>SFSQAVSGLNAAATNLDVIGNNIANSATYGFKSGTASFADMFAGSKVGLGVKVAGITQDFTDGTTTNTGRGLDVAISQNGFFRLVDSNGSVFYSRNGQFKLDENRNLVNMQGMQLTGYPATGTPPTIQQGANPAPITIPNTLMAAKSTTTASMQINLNSTDPVPSKTPFSVSDADSYNKKGTVTVYDSQGNAHDMNVYFVKTKDNEWAVYTHDSSDPAATAPTTASTTLKFNENGILESGGTVNITTGTINGATAATFSLSFLNSMQQNTGANNI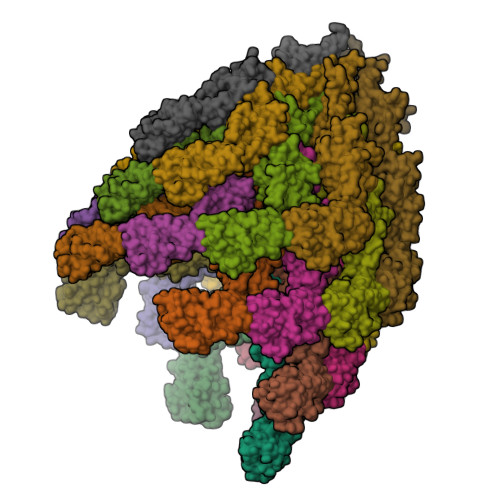VATNQNGYKPGDLVSYQINNDGTVVGNYSNEQEQVLGQIVLANFANNEGLASQGDNVWAATQASGVALLGTAGSGNFGKLTNGALEASNVDLSKELVNMIVAQRNYQSNAQTIKTQDQILNTLVNLR[26x]> GFPCGESCVYLPCFTAA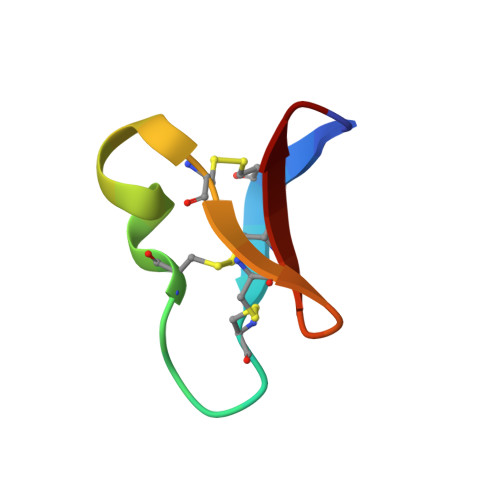IGCSCKSKVCYKN>SLFRTSPEMVQASLGETVKLRCEVMHSNTLTSCSWLYQKPGAASKPIFLMYLSKTRNKTAEGLDTRYISGYKANDNFYLILHRF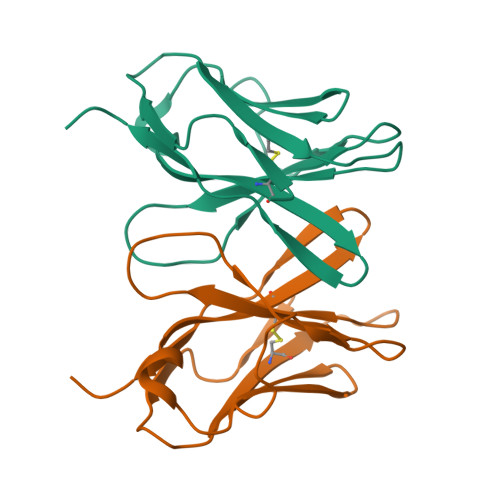REEDQGYYFCSFLSNSVLYFSNFMSVFLPA[2x]>[2x]GDIVSEKKPATEVDPTHFEKRFLKRIRDLGEGHFGKVELCRYDPEGDNTGEQVAVKSLKPESGGNHIADLKKEIEILRNLYHENIVKYKGICTEDGGNGIKLIMEFLPSGSLKEYL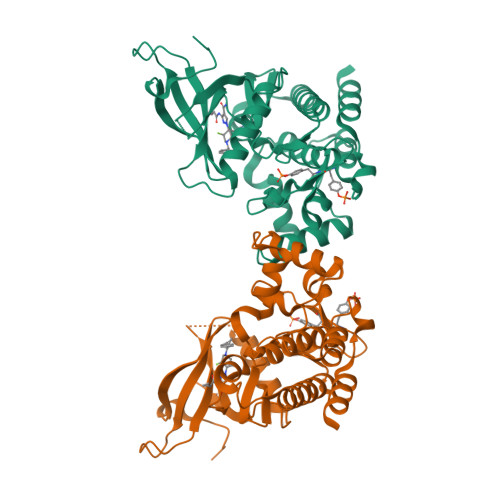PKNKNKINLKQQLKYAVQICKGMDYLGSRQYVHRDLAARNVLVESEHQVKIGDFGLTKAIETDKEYYTVKDDRDSPVFWYAPECLMQSKFYIASDVWSFGVTLHELLTYCDSDSSPMALFLKMIGPTHGQMTVTRLVNTLKEGKRLPCPPNCPDEVYQLMRKCWEFQPSNRTSFQNLIEGFEALLK tert-butyl {(2R,4S,6S,12Z,13aS,14aR,16aS)-2-[(7-chloro-4-methoxyisoquinolin-1-yl)oxy]-14a-[(cyclopropanesulfonyl)carbamoyl]-5,16-dioxo-1,2,3,5,6,7,8,9,10,11,13a,14,14a,15,16,16a-hexadecahydrocyclopropa[e]pyrrolo[1,2-a][1,4]diazacyclopentadecin-6-yl}carbamate | C36 H46 Cl N5 O9 S | 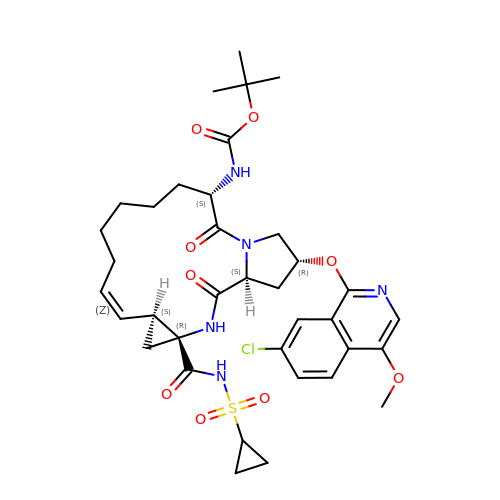ZFAXEHOMXOFIQU-HGSGLVRESA-N> NNEIMPGKM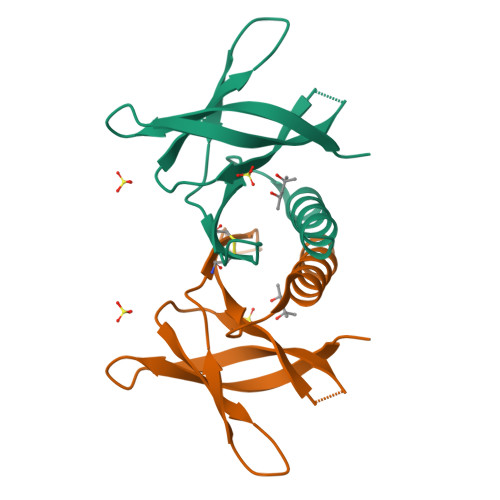KVKATKGEGDGGITSEGNALYNNEGGRAFMYAYVTTKPGMKYVKWEHDSGVVTVELEPPCRFVIDTPTGPQIKYLYFVKNLNNLRRGAVLGYIGATVRLQ>GAMPHDPSFTPTQLAARAAYLLRGNDLGTMTTAAPLLYPHMWSWDAAFVAIGLAPLSVERAVVELDTLLSAQWRNGMIPHIVFANGVDGYFPGPARWATATLADNAPRNRLTSGITQPPVHAIAVQRILEHARTRGRSTRAVAEAFLDRRWGDLMRWHRWLAECRDRNERGRITLYHGWESGMDNSPRWDSAYANVVPGKLPEYQRADNVIITDPSQRPSDGEYDRYLWLLEEMKAVRYDDERLPSVMSFQVEDVFFSAIFSVACQVLAEIGEDYKRPHADVKDLYLWAERFRAGVVETTDQRTGAARDFDVLAEKWLVTETAAQFAPLLCGGLPHDRERALLKLLEGPRFCGHPDLKYGLIPSTSPVSRDFRPREYWRGPVWPVLTWLFSWCFARRGWAERARLLRQEGL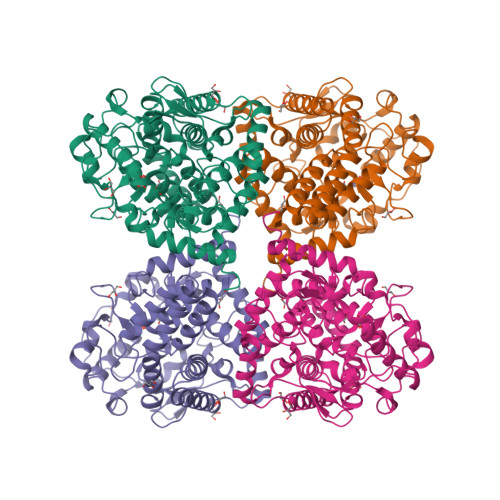RQASDGSFAEYYEPFTGEPLGSMQQSWTAAAVLDWLG[2x]TodS/TodT, a two-component signal transduction system, is responsible for regulation of tod operon expression in P. putida strains. TodS lacks a transmembrane region, and its N-terminal PAS domain (PAS1) binds a wide range of effectors, including toluene, to trigger increased basal autophosphorylation of TodS, leading to a phospho-signal relay to TodT and ultimately transcriptional stimulation of the tod operon genes by interacting with phosphorylated TodT in the PtodX promoter region (11–14). In the present study, we determined the crystal structures of the TodS PAS1 domain in complex with either toluene (an agonist) or 1,2,4-trimethylbenzene (1,2,4-TMB; an antagonist), as well that of apo-PAS1. The structure of each PAS1 domain is very similar to those described for other PAS domain structures, which consist of a five-stranded antiparallel β-sheet and three α-helices spanning residues 45–149.

We further determined the structure of PAS1 in complex with the antagonist 1,2,4-TMB. The same amino acid residues as those in the hydrophobic pocket are involved in the interaction with the antagonist. The only difference between PAS1 interactions with the agonist and those with the antagonist was found at the Phe46 position. The aromatic ring of the residue in complex with the antagonist is tilted ∼80° relative to that of Phe46 in complex with toluene in both molecules A and B (see “Discussion” for details). In molecule A, the Phe46 aromatic ring is tilted ∼80° in response to the antagonist 1,2,4-TMB relative to that of Phe46 either in apo-PAS1 or in complex with toluene. This change led to the formation of a salt bridge between two amino acid residues, Arg148 and Glu146, on the β5 strand, whereas no such bridge was observed in either apo- or agonist-bound PAS1. In the case of the antagonist 1,2,4-TMB, the equivalent region is completely disordered, and there was no electron density for amino acid residues after Lys155 in molecule B. Interestingly, residue Arg148 in molecule B of PAS1 complexed with the antagonist 1,2,4-TMB is very flexible and shows no visible electron density, whereas the electron density map of the corresponding residues in other structures is seen clearly. The phenomenon is probably related to the flexibility and lack of electron density in the STR region of molecule B of PAS1 complexed with 1,2,4-TMB. The ligand-dependent conformational change of TodS was also supported by the changed overall features of TodS complexed with the antagonist 1,2,4-TMB, which showed mainly oligomerization (bottom).

>GAMALYEFVGLLDAHGNVLEVNQVALEGGGITLEEIRGKPFWKARWWQISKKTEATQKRLVETASSGEFVRCDVEILGKSGGREVIAVDFSLLPICNEEGSIVYLLAEGRNITDKKKAEAMLALKNQELE[2x]1-(3-chlorophenyl)-3-{5-[2-(thieno[3,2-d]pyrimidin-4-ylamino)ethyl]-1,3-thiazol-2-yl}urea 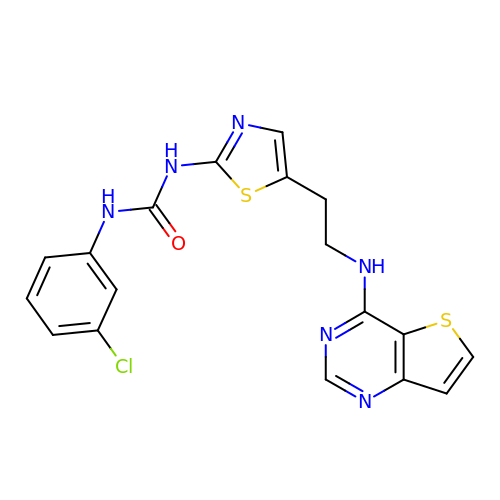| C18 H15 Cl N6 O S2 | FAYAUAZLLLJJGH-UHFFFAOYSA-N>GMSQMSPGQARVVDPILSTHARGYRQSTLIGKKLFPVAPVAQYGGKILTFGKEAFRLYNTKRAPGANTKRIDFGYEGDPYSIVPSALEAKVPRELMRDASQVPGIDLGARSVNTVLRIMALAHEHECAQIALDPAKYNADHKVKLVGSA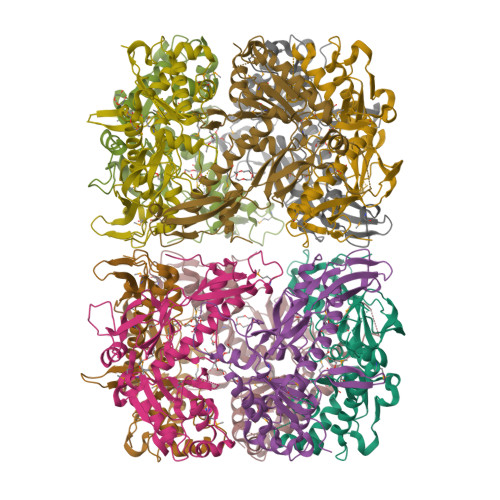RWTSPDSDPTKDVETAKEAIADSIGMEPNRLMLSRKALSACKYHPKLIERVKYTRAESITIDMLKALWEVEEIVVGTARVATGANDSFGDVWGPDVWLGYVSDNPDPSVEEPSFGYTYQIEGHPLVEVPYWDNNAKSWIYGVSDDNTPALSGMLAGYLIEDAGLPAA[10x]> AYFQGMVDVAFVCLGNICRSPMAEAIMRQRLKDRNIHDIKVHSRGTGSWNLGEPPHEGTQKILN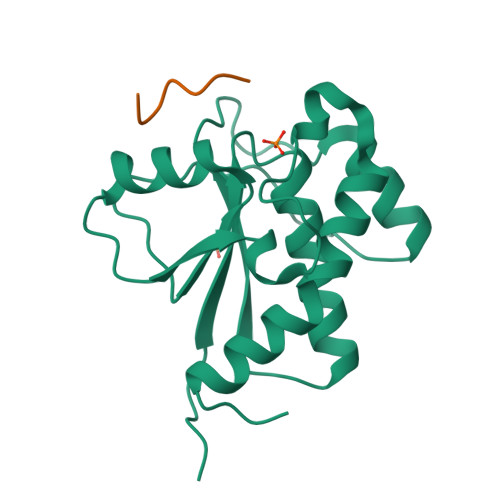KHNIPFDGMISELFEATDDFDYIVAMDQSNVDNIKSINPNLKGQLFKLLEFSNMEESDVPDPYYTNNFEGVYDMVLSSCDNLIDYIVKDANLKG;> HHHHHGS~{N}-[3-oxidanylidene-3-[[(1~{R})-1,2,3,4-tetrahydronaphthalen-1-yl]amino]propyl]-4-(trifluoromethyloxy)benzamide 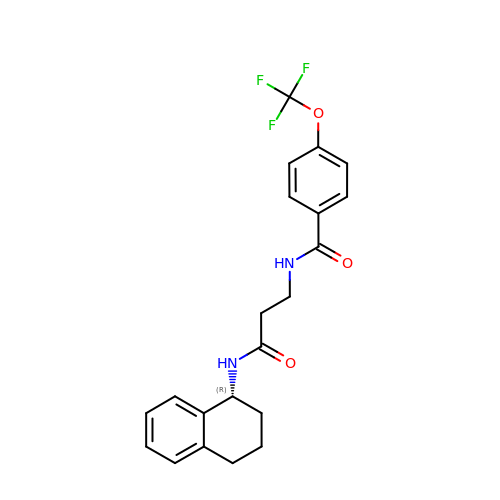| C21 H21 F3 N2 O3 | SGNRHEDBLPGDDC-GOSISDBHSA-N> ACPAPPPGQPDIRAIGYYTDKAGSVIDPALQQQNKDATAPLDRYAADVARMSDDYLRNGDPAAAQCTLSWLGAWADDGAM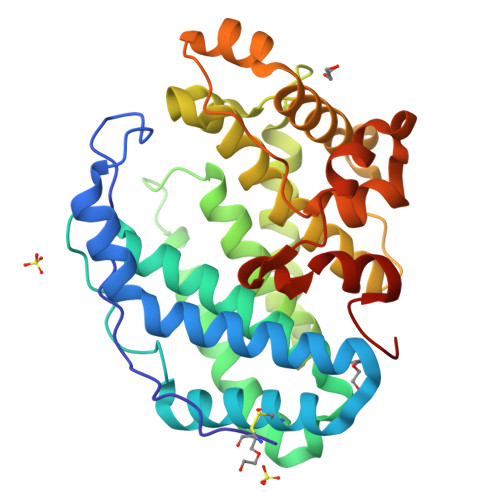LGQMIRVNNDQSFYMRQWMLDAVAMAYLKVHDQANPQQRARIDPWLQKLARANLAYWDNPKRRRNNAYYWGGLGVLATGLATDDDALWQAGHAAFQKGIDDIQDDGSLPLEMARGQRALHYHDYALAPLVMMAELARLRGQDWYASRNHAIDRLARRVIEGSRDPAWFNQHTGAAQLPLQASGWVEFYRLRSPDGGVFDAAHARGPFHSPRLGGDLTLMATHGIVRTPLRHHHHHH> SMGIHATEELKEFFAKARAGSVRL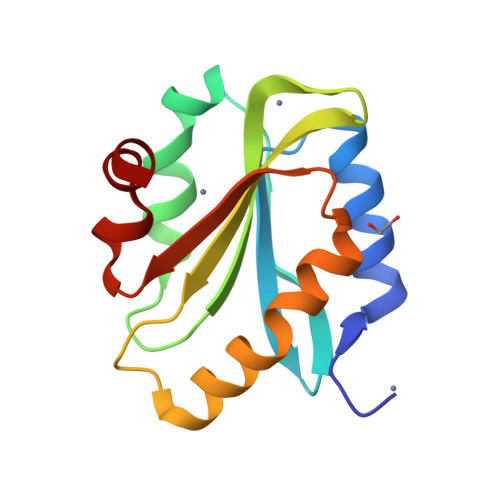IKVVIEDEQLVLGASQEPVGRWDQDYDRAVLPLLDAQQPCYLLYRLDSQNAQGFEWLFLAWSPDNSPVRLKMLYAATRATVKKEFGGGHIKDELFGTVKDDLSFAGYQKH>[3x]ARKGKKTNSNQGQQGKRKSRRPRGRSAEPQLQRAPVAQAS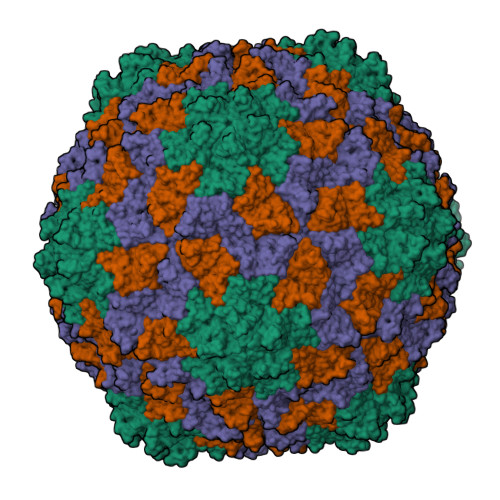RISGTVPGPLSSNTWPLHSVEFLADFKRSSTSADATTYDCVPFNLPRVWSLARCYSMWKPTRWDVVYLPEVSATVAGSIEMCFLYDYADTIPRYTGKMSRTAGFVTSSVWYGAEGCHLLSGGSARNAVVASMDCSRVGWKRVTSSIPSSVDPNVVNTILPARLAVRSSIKPTVSDTPGKLYVIASMVLRDPVDPTLNT> MAVKPMLHYFNGRGRMEPIRWLLAAAGVEFEETFIDTPEDFEKLKNDGSLMFQQVPMVEIDGMKLVQSRAILNYVAAKHNLYGKDIKERALIDMYIEGVADLNEMILLLPITPPAEKD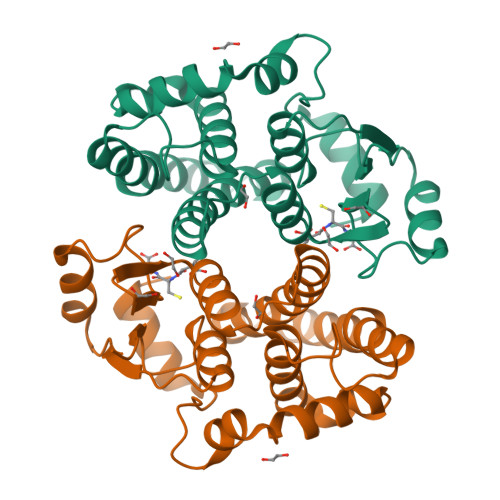AKIMLIKDRTTNRYLPAFEKVLKSHGEDYLVGNRLSRADIHLVELLYLVEELDPSLLTNFPLLKALKARISNLPTVKKFLQPGGARKPPGDEKSVEKSRKIFKF> MAFRSANTRATNVVNYAANQSGRNVNHLVFANTSYEILGGGKKYNQVFMTMDGKLKIKIDYTVDDSVVEGDYFTVDFGKYIHPGTSRKPYRVNNIHDANGRTIAIGSYDSATNTAKYTFTNYVDIYNNVRGSFSLLSWPFKELVTTDKQSVPVGITVAGEDYTQNVIFNYGNRTVPVISDINYLTKDFAEFTTYINQNRAFNTGSKVRLSGQGFKFTSPDEIEVYKVLNNSQFRDSFSPDYANLTQVRNPKIIINSDGSATVDLGDIGTLGYIIRSKPNTLPDFSGIGVLKSEYTFTNNKNQRDTRAHASSIQFVRAELAGFGGFGGYVWFDKNNDGVQNDSNAAAAGITVNLLDPTGIRLATTTTDITGHYNFDNLTNGNYLVEFVMPEGYIPTQANSTVDDKDSDVVFENGRYIAHVTIKDADNMTIDAGLVSD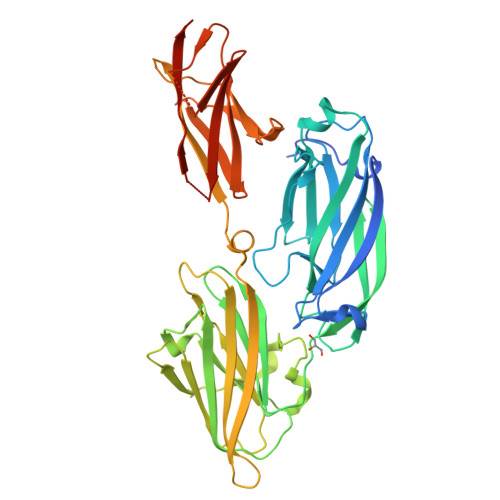TTLEHHHHHH>GPAMATNGEIFNTYGHNHQSATVTKITASNESSNGVCYLSETANLGKLICIPMALRAAMELNVFQLISKFGTDAKVSASEIASKMPNAKNNPEAAMYLDRILRLLGASSILSVSTTKKSINRGGDDVVVHEKLYGLTNSSCCLVPRQEDGVSLVEELLFTSDKVVVDSFFKLKCVVEEKD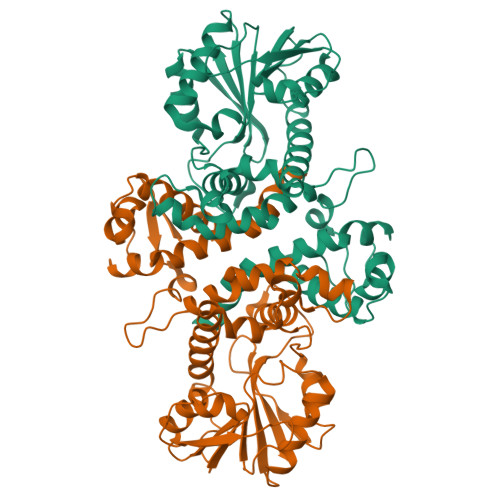SVPFEVAHGAKIFEYAATEPRMNQVFNDGMAVFSIVVFEAVFRVYDGFLDMKELLDVGGGIGTSVSKIVAKYPLIRGVNFDLPHVISVAPQYPGVEHVAGDMFEEVPKGQNMLLKWVLHDWGDERCVKLLKNCWNSLPVGGKVLIIEFVLPNELGNNAESFNALIPDLLLMALNPGGKERTISEYDDLGKAAGFIKTIPIPISNGLHVIEFHK[4x]(1R,2S,3S,4R,6S)-4,6-diamino-3-{[3-deoxy-4-C-methyl-3-(methylamino)-beta-L-arabinopyranosyl]oxy}-2-hydroxycyclohexyl 2-amino-2,3,4,6-tetradeoxy-6-[({3-hydroxy-2-methyl-5-[(phosphonooxy)methyl]pyridin-4-yl}methyl)amino]-beta-L-threo-hexopyranoside 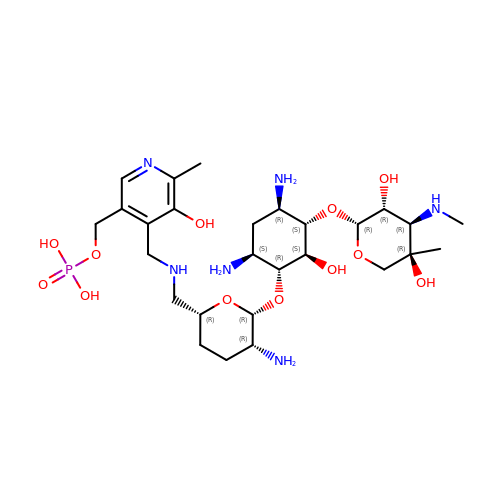| C27 H49 N6 O12 P | RIDGEVUBNCTQEZ-LVJYRULHSA-N> MAYIAVPAVVDSRSSEAIGLLESFGVDAGADANDVSYQDHDYVLDQLQYMLDGYEAGDVIDALVHKNWLHHSVYCLLPPKSQLLEYWKSNPSAIPDNVDRRLRKRLMLKKDLRKDDEYNQLARAFKISDV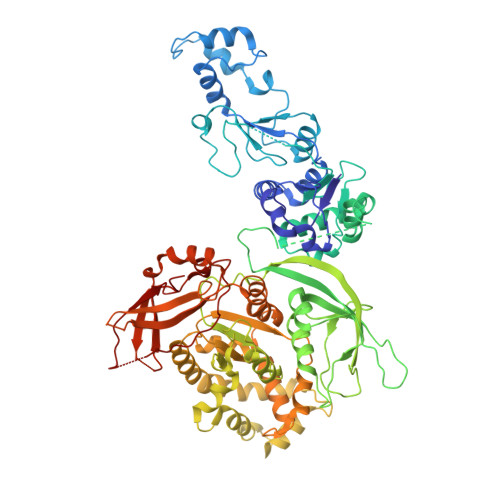YAPLISSTTSPMTMIQNLNQGEIVYTTTDRVIGARILLYAPRKYYASTLSFTMTKCIIPFGKEVGRVPHSRFNVGTFPSIATPKCFVMSGVDIESIPNEFIKLFYQRVKSVHANILNDISPQIVSDMINRKRLRVHTPSDRRAAQLMHLPYHVKRGASHVDVYKVDVVDMLFEVVDVADGLRNVSRKLTMHTVPVCILEMLGIEIADYCIRQEDGMLTDWFLLLTMLSDGLTDRRTHCQYLINPSSVPPDVILNISITGFINRHTIDVMPDIYDFVKPIGAVLPKGSFKSTIMRVLDSISILGIQIMPRAHVVDSDEVGEQMEPTFEQAVMEIYKGIAGVDSLDDLIKWVLNSDLIPHDDRLGQLFQAFLPLAKDLLAPMARKFYDNSMSEGRLLTFAHADSELLNANYFGHLLRLKIPYITEVNLMIRKNREGGELFQLVLSYLYKMYATSAQPKWFGSLLRLLICPWLHMEKLIGEADPASTSAEIGWHIPREQLMQDGWCGCEDGFIPYVSIRAPRLVIEELMEKNWGQYHAQVIVTDQLVVGEPRRVSAKAVIKGNHLPVKLVSRFACFTLTAKYEMRLSCGHSTGRGAAYSARLAFRSDLA> GMNPENWLLLRRVVRFGDTDAAGVMHFHQLFRWCHESWEESLESYG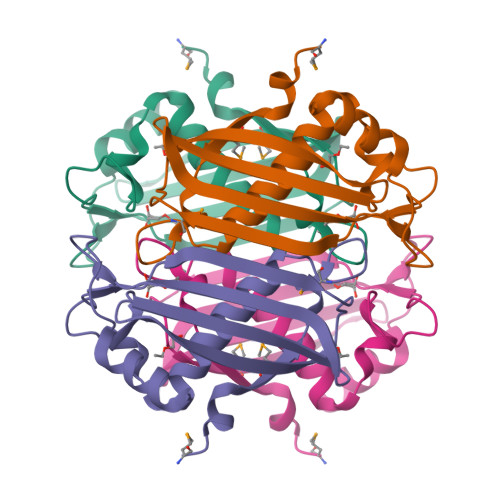LNPADIFPGSRKSEVTPEVALPIIHCQADFRRPIHTGDALAMELRPERLNPNSFQVHFEFRCEEQIAAHALIRHLAINAQTRHRCALPEGIDRWLEASGVGKIGSI>[2x]MEMMIKKRIKQVKKGDQDAFADIVDIYKDKIYQLCYRMLGNVHEAEDIAQEAFIRAYVNIDSFDINRKFSTWLYRIATNLTIDRIRKKKPDYYLDAEVAGTEGLTMYSQIVADGVLPEDAVVSLELSNTIQQKILKLPDKYRTVIVLKYIDELSLIEIGEILNIPVGTVKTRIHRGREALRKQLRDL;>[2x]MSCPEQIVQLMHMHLDGDILPKDEHVLNEHLETCEKCRKHFYEMEKSIALVRSTSHVEAPADFTANVMAKLPKEKKRASV

SigW is one of ECF sigma factors in the gram-positive model bacterium Bacillus subtilis. Its activity is suppressed by the anti-sigma RsiW under normal growth conditions. The cytoplasmic domain (RsiWcyto) interacts tightly with SigW to inhibit SigW activity. In the structure, RsiWcyto interacts with the groove formed along the surface of two domains in SigW (σW2 and σW4), resulting in the burial of the promoter binding area of SigW.

Rod-shaped crystals grown in the condition containing polyethylene-glycol 3350 as a precipitant diffracted up to 2.8 Å resolution. Thus, the structure was determined by the multi-wavelength anomalous dispersion (MAD) method, using a crystal of selenomethionine-labeled SigW/RsiWcyto. The residues of two SigW/RsiWcyto complexes in the asymmetric unit (residues 3-95 and 125-187 in SigW and residues 3-72 in RsiW) were traced into the electron density and the final model was refined with R/Rfree values of 21.0/28.7%. Two SigW/RsiWcyto complexes in the asymmetric unit are superimposed with a root-mean-square deviation (rmsd) of 0.7 Å for 224 Cα atoms, indicating that the two complexes have the same conformation. The x-ray emission spectrum measured in the synchrotron facility revealed that the crystal contains zinc ion bound to SigW/RsiWcyto. In the structure of RsiWcyto, the zinc ion is coordinated by residues C3 in L1’, H30 in α2’, C34 in L3’, and C37 in α3’. The three N-terminal alpha-helices (α1’-α3’) form a helical bundle and coordinate a zinc ion. By contrast, RsiWcyto interacts with SigW by wrapping the surface of SigW, resulting in a large surface burial of 3324 Å2. The surface binding area of SigW/RsiWcyto is divided into three binding motifs of RsiWcyto. Taken together, anti-sigma RsiW inhibits the promoter binding of SigW by directly blocking the binding surface of -35 element in σW4.>GSHMTQDCSFQHSPISSDFAVKIRELSDYLDQDYPVTVASNLQDEELCGGLWRLVLAQRWMERLKTVAGSKMQGLLERVNTEIHFVTKCAFQPPPSCLRFVQTNISRLLQETSEQLVALKPWITRQNFSRCLELQCQP[2x]

FLT3 is a transmembrane receptor that is expressed on the surface of early hematopoietic progenitor cells and dendritic cells. Mature wild-type FL belongs to the structural family of short-chain four-helical bundle cytokines and consequently exhibits a noncovalently linked homodimeric structure, in which the two protomers interact head to head. Due to their highly similar build and the dimeric nature of their cognate cytokine ligands, RTK-IIIs are thought to be activated by similar mechanisms. The binding of a dimeric cytokine to an RTK-III induces receptor dimerization that results in transactivation of the auto-inhibited tyrosine kinase domains and the activation of downstream signaling pathways. However, structural studies have shown that the hematopoietic receptor FLT3, a class III RTK, does not appear to engage in such receptor–receptor contacts, despite its efficient dimerization by dimeric FLT3 ligand (FL).

As part of efforts to better understand the intricacies of FLT3 activation, we sought to engineer a monomeric FL. It was found that a Leu27Asp substitution at the dimer interface of the cytokine led to a stable monomeric cytokine (FLL27D) without abrogation of receptor binding. By mutating Leu27 to an aspartate, we hypothesized that the entropic penalty for burying a charged residue in the hydrophobic interior of the second protomer would be detrimental for any dimerization event to occur. We concluded that these experimentally determined values are in excellent agreement with their theoretical molecular weights and confirmed that FLL27D is indeed a monomeric species in solution. With only an excess of FLL27D detected, this shift indicates that despite its monomeric nature, FLL27D was still able to recruit all available receptor molecules into complex formation. The molecular species has a molecular mass of 70 kDa as determined by SEC-MALLS, which is well below that of an FL-mediated receptor complex (152 kDa) and therefore allowed us to infer that the apparent FLL27D–FLT3 complex consists of one molecule of FLL27D and one molecule of FLT3. Given the observation that FLL27D still binds FLT3, it comes as no surprise that the absence of structural deviation from FLWT remains valid for residues 6–13, which are all key players in the largest interaction site of the FL–FLT3 epitope. Importantly, although the triclinic unit cell contains two copies of FLL27D with apparent twofold rotational symmetry, the observed apparent symmetry axis is dramatically distinct in direction and context from the twofold-symmetry axis in dimeric FLWT. Likewise, no combination of symmetry relations can reconstitute the head-to-head dimer resembling FLWT, despite the fact that the loop containing Asp27 is located near tightly packed crystal lattice contacts.> MGSSHHHHHSSGENLYFQGHMGKYTKKFNEVRSTDRPLVGGKCASLGEMVQAGLPVPDGFAVTIDAYEDFRDDSDLRAELRSLVFGVDPDSSKSLQDAHDQAVALVLGRNLPAAIEDEIREAYLTLSRETARRRGTGDTDRIPVAVRSSSVDEDGDAASFAGQQETYLWVVGADDVIAKVRECWASLYTPQAIAYRAGMSETDAAEASKISVAVQLMADADVAGVMFTVSPRTGDRSVIAINASWGLGQSVVSGEVTPDEYWLSKIGPTLTSSRIASKEHEYVPAPDGTGVIFREVEQARREVSCLSDSELMQLAEIGLRVEEHYGCPQDIEWALEHDSDGTSRVMLLQSRPETNWKKRKEEKSKRTSSATSNLLGFVSAAAKGQTR

Catabolism in GD02 is initiated by a two-component kinase, HpeHI, which catalyzes the ATP-dependent phosphorylation of AV or HAP to 4-phospho-AV or 4-phosphoacetophenone (PAP), respectively. The structural data indicate that HpeHI is a two-component homolog of RPH, a single component enzyme involved in antibiotic resistance.

Crystals of HpeI diffracted to 1.8 Å resolution, and the structure was solved by molecular replacement using an HpeI AlphaFold model (AF-A0A520FAS4-F1-v4), with the N- and C-terminal lobes as separate search models. The ATP-binding site is located at the interface between the N- and C-terminal α/β lobes. The motif comprises β-strands 3 and 4 and their joining loop (V124-V150) located in the N-terminal α/β lobe. The motif from all phenolic substrate kinases more closely resembles PEP synthase than PPDK. Notably, residues 133 to 142 comprising the conserved loop could not be modeled in our HpeI structure and are presumably disordered. Another notable feature of the HpeI structure is that it is in a more open conformation than many characterized grasp domains. The ATP grasp domains from RPH and PPDK structures were shown to undergo a hinge-like ATP-dependent conformational change between the two α/β lobes to enclose ATP. Given that HpeI was crystallized in the absence of ATP, the crystals likely represent the open conformation, and it would similarly undergo ATP-dependent closure upon binding, though no crystals of the nucleotide-bound form were obtained. More particularly, the structural data indicate that HpeI corresponds to the ATP-grasp domain of RPH while HpeH harbors the swivel and RIF-binding domains of RPH.>MAYSQGGGKKKVCYYYDGDIGNYYYGQGHPMKPHRIRMTHNLLLNYGLYRKMEIYRPHKATAEEMTKYHSDEYIKFLRSIRPDNMSEYSKQMQRFNVGEDCPVFDGLFEFCQLSTGGSVAGAVKLNRQQTDMAVNWAGGLHHAKKSEASGFCYVNDIVLAILELLKYHQRVLYIDIDIHHGDGVEEAFYTTDRVMTVSFHKYGEYFPGTGDLRDIGAGKGKYYAVNFPMRDGIDDESYGQIFKPIISKVMEMYQPSAVVLQCGADSLSGDRLGCFNLTVKGHAKCVEVVKTFNLPLLMLGGGGYTIRNVARCWTYETAVALDCEIPNELPYNDYFEYFGPDFKLHISPSNMTNQNTPEYMEKIKQRLFENLRMLPHAPGVQMQAIP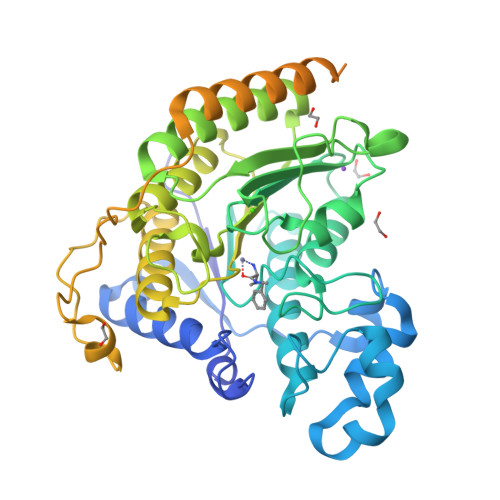EDAVHEDSGDEDGEDPDKRISIRASDKRIACDEEFSDSEDEGEGGRRNVADHKKGAKKARIEEDKKETEDKKTDVKEEDKSKDNSGEKTDTKGTKSEQLSNPGSSGHHHHHH[3x]> S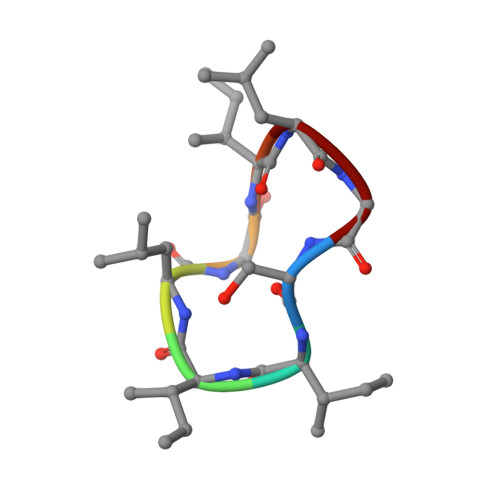IILGILG> MASMTGGQQMGRGSS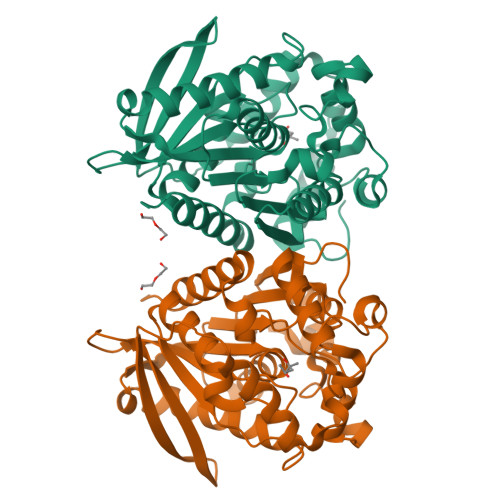GSPGVEQHTQAFLEALEQGGGKPLEQLSPKDARAVLTGAQASVKVDLSGIEVKERTIQANGQSIKLQVVRPANVKGELPVFMFFHGGGWVLGDFPTHQRLIRDLVVGSGAVAVYVDYTPSPESHYPTAINQAYAATQWVAEHGKEIGVDGKRLAVAGNSVGGNMAAVVALKAKEAGTPALRFQLLLHPVTDASFETASYKQFADGHFLTTGMMKWFWDNYTTDAKAREQIYASPLRASSEQLKGLPPALVQTAEFDVLRDEGEAYARKLNAAGVTVTSVRYNGMIHDYGLLNPLSQVPAVKAAMRQAGTELKVHLQLELEHHHHHH> GDPIADMIDQTVNNQVNRSLTALQVLPTAANTEASSHRLGTGVVPALQAAETGASSNASDKNLIETRCVLNHHSTQETAIGNFFSRAGLVSIITMPTTGTQNTDGYVNWDIDLMGYAQLRRKC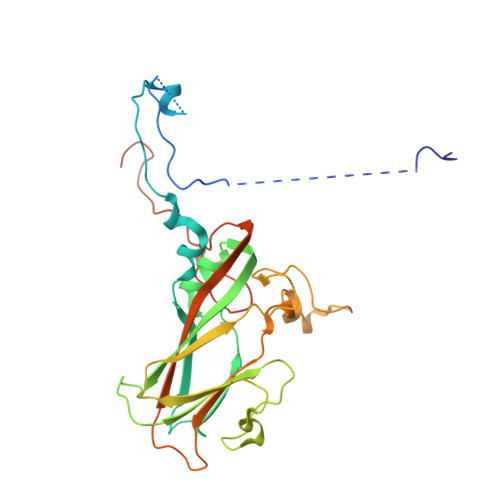ELFTYMRFDAEFTFVVAKPNGELVPQLLQYMYVPPGAPKPTSRDSFAWQTATNPSVFVKMTDPPAQVSVPFMSPASAYQWFYDGYPTFGEHLQANDLDYGQCPNNMMGTFSIRTVGTEKSPHSITLRVYMRIKHVRAWIPRPLRNQPYLFKTNPNYKGNDIKCTSTSRDKITTL>[2x]ESSRSAMMYIQELRSGLRDMHLLSCLESLRVSLNNNPVSWVQTFGAEGLASLLDILKRLHDEKEETSGNYDSRNQHEIIRCLKAFMNNKFGIKTMLETEEGILLLVRAMDPAVPNMMIDAAKLLSALCILPQPEDMNERVLEAMTERAEMDEVE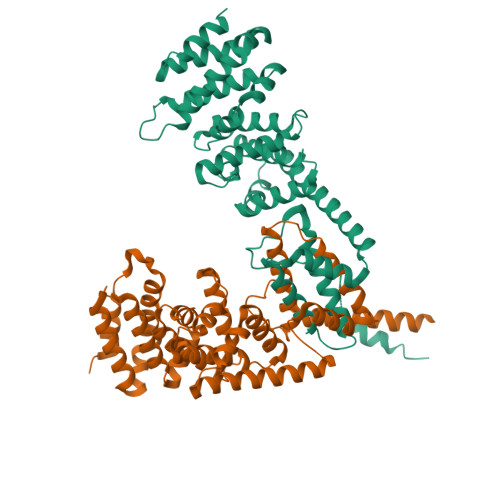RFQPLLDGLKSGTSIALKVGCLQLINALITPAEELDFRVHIRSELMRLGLHQVLQELREIENEDMKVQLCVFDEQGDEDFFDLKGRLDDIRMEMDDFGEVFQIILNTVKDSKAEPHFLSILQHLLLVRNDYEARPQYYKLIEECVSQIVLHKNGTDPDFKCRHLQIDIERLVDQMIDKTKVEKSEAKATELEKKLDSELTARHELQVEMKKMENDFEQKLQDLQGEKDALDS> GSGNSHTTPWTNPGLAENFMNSFMQGLSSMPGFTASQLDDM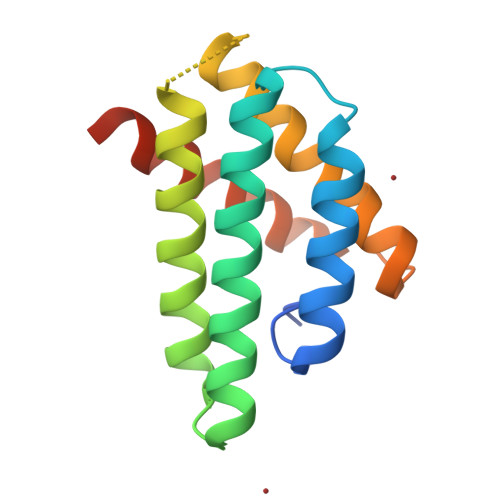STIAQSMVQSIQSLAAQGRTSPNKLQALNMRFASSMAEIAASEEGGGSLSTKTSSIASAMSNAFLQTTGVVNQPFINEITQLVSMFAQAGMNDVSA>MSEYIRVTEDENDEPIEIPSEDDGTVLLSTVTAQFPGACGLRYRNPVSQCMRGVRLVEGILHAPDAGWGNLVYVVNYPKDNKRKMDETDASSAVKVKRAVQKTSDLIVLGLPWKTTEQDLKEYFSTFGEVLMVQVKKDLKTGHSKGFGFVRFTEYETQVKVMSQRHMIDGRWCDCKLPNSKQSQDEPLRSRKVFVGRCTEDMTEDELREFFSQYGDVMDVFIPKPFRAFAFVTFADDQIAQSLCGEDLIIKGISVHISNAEPKHNSNRQLERSGRFGGNPGGFGNQGGFGNSRGGGAGLGNNQGSNMGGGMNFGAFSINPAMMAAAQAALQSSWGMMGML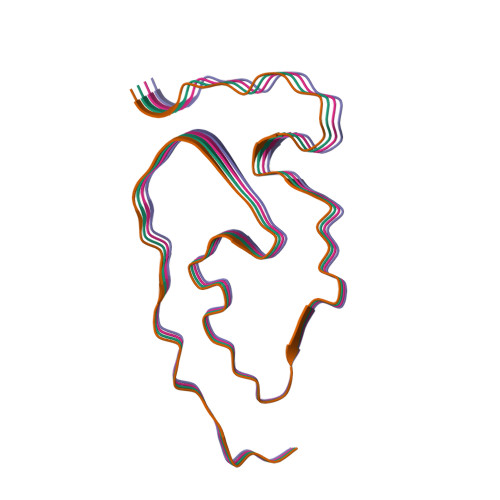ASQQNQSGPSGNNQNQGNMQREPNQAFGSGNNSYSGSNSGAAIGWGSASNAGSGSGFNGGFGSSMDSKSSGWGM[4x]> GPEFVSFANQLQALGLKLREVPGDGNCLFRALGDQLEGHSRNHLKHRQETVDYMIKQREDFEPFVEDDIPFEKHVASLAKPGTFAGNDAIVAFARNHQLNVVIHQLNAPLWQIRGTEKSSVRELHIAYRYGEHYDSVRRINDNS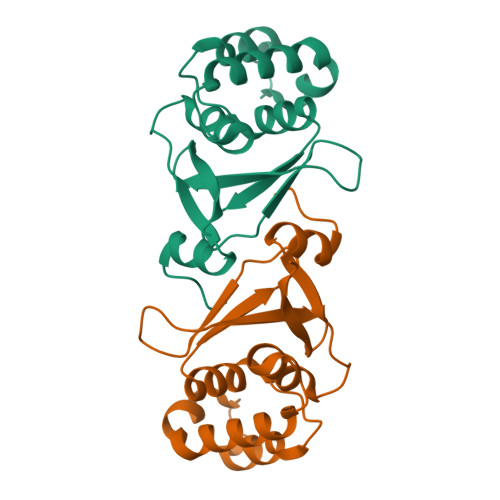EAPAHLQTDFQMLHQD>MAPLRKTYVLKLYVAGNTPNSVRALKTLNNILEKEFKGVYALKVIDVLKNPQLAEEDKILATPCLAKVLPPPVRRIIGDLSNREKVLIGLDLLYE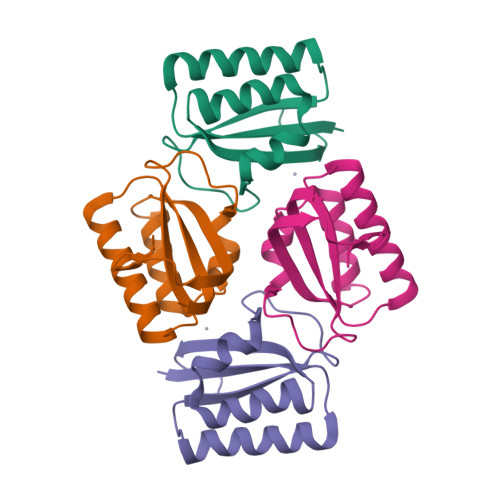EIGDQAEDDLGLE[4x]WXG100 proteins are a group of proteins of approximately ∼100 residues in length that contain a conserved “Trp-Xaa-Gly (WXG)” motif. To investigate how specific sequence motifs translate into specific structural features, we determined the atomic structures of two representative complexes, the heterodimeric CFP-10/ESAT-6 complex and the homodimeric sagEsxA assembly. The overall structures of the two protein complexes are similar, with both forming a four-helix bundle, in which each monomer consists of a helix-loop-helix structural motif. However, the novelty of this contribution is that by using the iterative bio-informatics approach, we can show that the WXG100 protein superfamily can be divided into three subfamilies: CFP-10-, ESAT-6- and sagEsxA-like.

The sagEsxA-like proteins form a homodimer and the structure of the sagEsxA shows that the driving force for the interdimer interactions is principally hydrophobic in nature. At the inter-dimeric interface, hydrophobic residues are prevalent in sagEsxA-like proteins although there is a pair of hydrophilic residues Y18 and Q36 within the hydrophobic core of sagEsxA. The side chains of these residues form hydrogen bonds within the hydrophobic core of the four-helix-bundle complex (inset) and the presence of these hydrogen bond pairs between Y18 and Q36 is indicative of the anti-parallel homodimer arrangement found in the sagEsxA subfamily of WXG100 proteins. As a result, this conserved pair of mutations can be seen as a fingerprint of anti-parallel homodimeric WXG100 proteins. Therefore, both the CFP-10 and sagEsxA loops are considerably more flexible, which is reflected by the presence of different conformations in each of the copies of the asymmetric units. The CFP-10 subfamily is structurally more closely related to the sagEsxA than to the ESAT-6 subfamily. This is reflected by a root mean square deviation (r.m.s.d) of 2.07 Å for a superimposition of the core residues of CFP-10 (residues 11–83) and sagEsxA (residues 11–83), compared to an r.m.s.d. of 3.43 Å for the equivalent ESAT-6/sagEsxA superimposition. Secondly, by examining every WXG100 gene in its genetic context we could clearly show that all WXG100 genes from the Actinobacteria phylum are encoded in a bi-cistronic operon containing a CFP-10-like gene followed by an ESAT-6-like gene without exception, whereas, all the sagEsxA-like genes occur as mono-cistronic genes in the bacterial genomes belonging to Firmicutes. Interestingly, the sagEsxA FRET signal could only be detected after extensive heat treatment. This result shows that the homodimer is stable, and a FRET pair homodimer can only be reconstituted after heat dissociation.

>[4x]GAMSQIKLTPEELRSSAQKYTAGSQQVTEVLNLLTQEQAVIDENWDGSTFDSFEAQFNELSPKITEFAQLLEDINQQLLKVADIIEQTDADIASQISG> KETAAAKFERQHMDSSTSAASSSNYCNQMMKSRNLTKDRCKPVNTFVHESLADVQAVCSQKNVACKNGQTNCYQSYSTMSATDCRETGSSKYPNCAYKTTQANKHIIVACEGNPYVPVH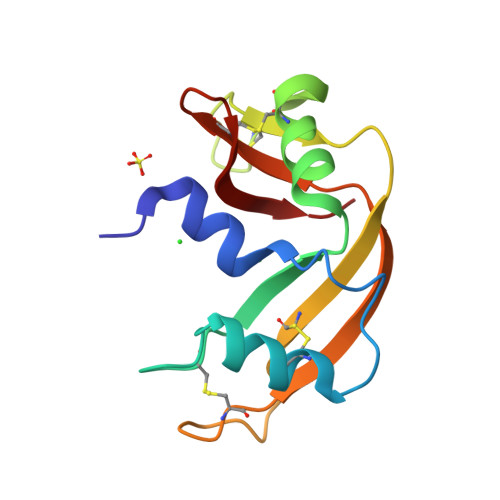FDASV>SRCTHLENRDFVTGVQGTTRLTLVLELGGCVTVTADGKPSLDVWLDSIYQESPAQTREYCLHAKLTGTKVAARCPTMGPATLPEEHQSGTVCKRDQSDRGWGNHCGLFGKGSIVTC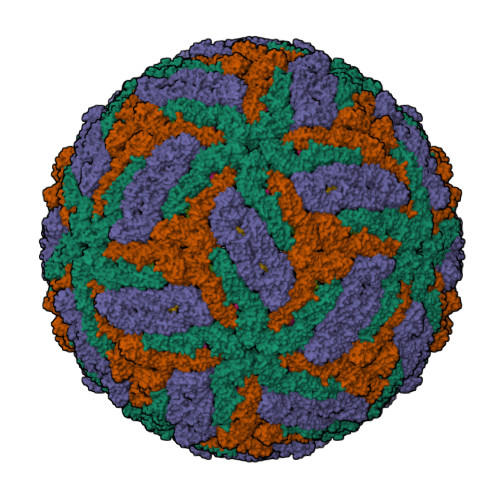VKFTCEDKKKATGHVYDVNKITYTIKVEPHTGEFVAANETHSGRKSASFTVSSEKTILTLGDYGDVSLLCRVASGVDLAQTVVLALDKTHEHLPTAWQVHRDWFNDLALPWKHDGAEAWNEAGRLVEFGTPHAVKMDVFNLGDQTGVLLKSLAGVPVASIEGTKYHLKSGHVTCEVGLEKLKMKGLTYTVCDKTKFTWKRAPTDSGHDTVVMEVGFSGTRPCRIPVRAVAHGVPEVNVAMLITPNPTMENNGGGFIEMQLPPGDNIIYVGDLNHQWFQKGSSIGRVLQKTRKGIERLTVLGEHAWDFGSVGGVMTSIGRAMHTVLGGAFNTLLGGVGFLPKILLGVAMAWLGLNMRNPTLSMGFLLSGGLVLAMTLGVGA[3x];>[3x]VLIPSHAQRDLTGRGHQWLEGEAVKAHLTRVEGWVWKNKLFTLSLVMVAWLMVDGLLPRILIVVVALALAPAYA> MLRT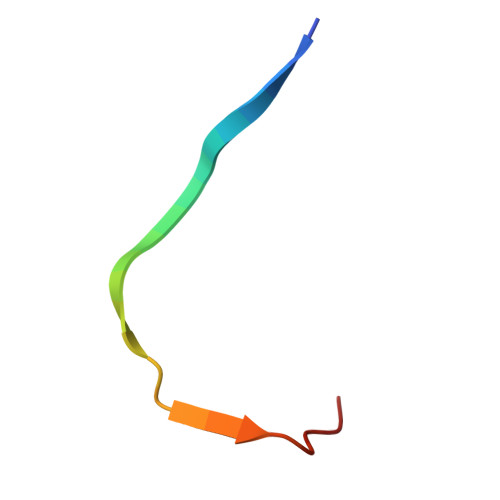MLKSKIHRATVTCADLHYVG2-methyl-1-[(2R)-2-oxidanylpropyl]-9H-carbazole-3,4-dione | C16 H15 N 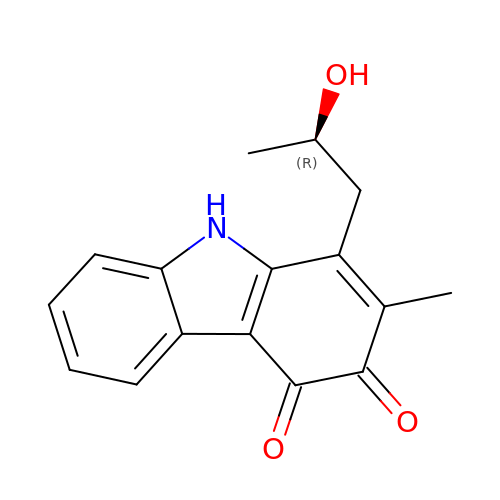O3 | HADDOKGXXGGODW-MRVPVSSYSA-N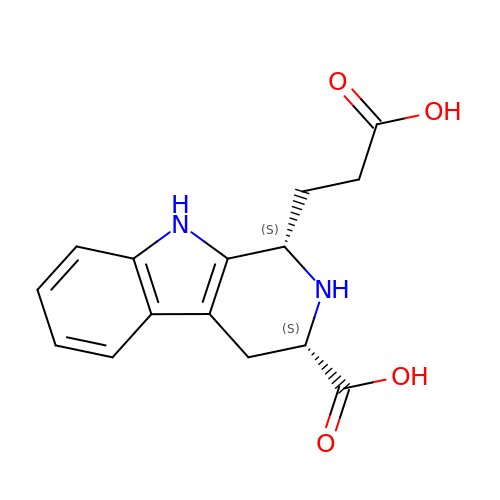(1S,3S)-1-(2-carboxyethyl)-2,3,4,9-tetrahydro-1H-pyrido[3,4-b]indole-3-carboxylic acid | C15 H16 N2 O4 | PPKGNUKJFFAWHY-RYUDHWBXSA-N> MQLTPTFYDNSCPNVSNIVRDTIVNELRSDPRIAASILRLHFHDCFVNGCDASILLDNTTSFRTEKDAFGNANSARGFPVIDRMKAAVESACPRTVSCADLLTIAAQQSVTLAGGPSWRVPLGRRDSLQAFLDLANANLPAPFFTLPQLKDSFRNVGLNRSSDLVALSGGHTFGKNQCRFIMDRLYNFSNTGLPDPTLNTTYLQTLRGLCPLNGNLSALVDFDLRTPTIFDNKYYVNLEEQKGLIQSDQELFSSPNATDTIPLVRSFANSTQTFFNAFVEAMDRMGNITPLTGTQGQIRLNCRVVNSNS

Of all the heme peroxidases, horseradish peroxidase (HRP) is arguably the most iconic. Heme peroxidase enzymes are highly proficient in oxidizing small aromatic substrates, but HRP is the most proficient with catalytic activities that far outpace other peroxidases. Such high activity, producing easily detectable coloured or fluorescent products, makes HRP a very sensitive diagnostic tool in a wide range of biotechnological assays. But the native enzyme, as isolated from horseradish roots, is heavily glycosylated which has hampered its successful crystallization for decades.

In this work, we produced recombinant HRP in E. coli and obtained an X-ray structure of the ferric enzyme at 1.63 Å resolution. The structure contains a total of 306 residues with 15 α-helices (148 residues) and 2 anti-parallel β-sheets (6 residues). HRP contains four disulphide bonds (between residues C11–C91, C44–C49, C97–C301, and C177–C209), which are highly conserved among the class III peroxidases and observed in our structure. Additionally, there are two calcium ions present in the structure, although not in the vicinity of the active site. The distance between the heme iron and the Nε atom of the proximal His 170 is 2.0 Å, while that between the heme iron and Nε of distal histidine (His 42) is 6.1 Å. An ethylene glycol (EDO) situated at the δ-heme edge of the active site is at 4.0 Å from iron (Fe–O2). Ethylene glycol does not interact with the heme iron, but potentially forms hydrogen bonds with the distal histidine (O2-Nε = 2.7 Å) and arginine (O2-Nε = 3.1 Å, O1-Nη = 3.0 Å) residues. There is no distal water molecule within the bonding distance of the iron on the distal side, and there is no ferulic acid binding at the δ-heme edge (as has been observed in previous HRP structures). Hence, multiple steps of crystallization may have led to the removal of ferulic acid from the HRP active site, which was occupied by ethylene glycol during cryoprotection.>[20x]TLIELMIVVAIIGILAAIAIPQYQNYIAKSQVSRVMSETGSLKTVIETCILDGKTAANCELGWTNSNLLG;>[20x]STAAVTGQTGLTITYPASATESAAIQGTFGNSAAIKIKNQTLTWTRTPEGAWSCATTVEAKFKPAGCAS;> MNMYKWVPESIRD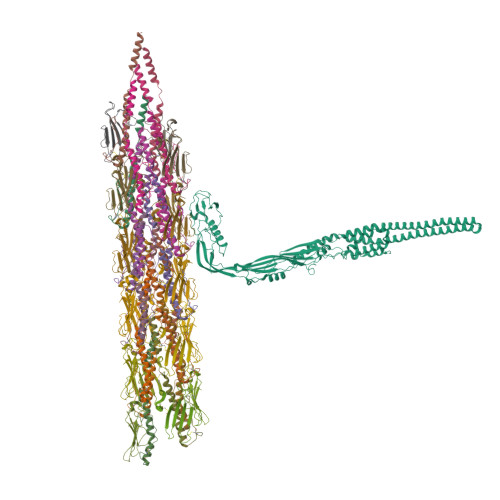SGEGQPSYSNNGDYAPSGPWVAAGIHTMPQSLRDSMRNSIMVTAQARRDVIGPEWGPDGRFTGYASVIGTPDPKPADIVNKFTVERRPVSNGNFQQRVKAGDIVVAPYTSDGKITVKLVAGQKDISSTPDYDYRIDSSLASSAGFVVAGERWYYTKRHFIIPRYFQNWRMRRRKYVTGWVMPTFYSPKEIFNRLKDSLVPDTGLVTQVWADNNTKRMDFLTAMAEIPQTLSSFLDALGYLGSLIKDFKRRRFFLNKAHQRIRNKLGVSFAERRSQIVSKYDRKIASARKPAIIVKLRQRKEKALKALDKMRVREEKKMIREFATQAASLWLSFRYEIMPLYYQSQDVLDVIANSTSEFMTSRDFVAKAINIGIPLEWNLDQENLVSQPRHNVMVKSKLSPENNIGKTLSVNPFTTAWELLTLSFVVDWFVNFGDVIAGFTGGYSDDSGATASWRFDDKKVFHLKNIPSAMVIVDINFYTRQVIDPRLCGGLAFSPKLNLFRYLDAMSLSWNRSRLKISRAT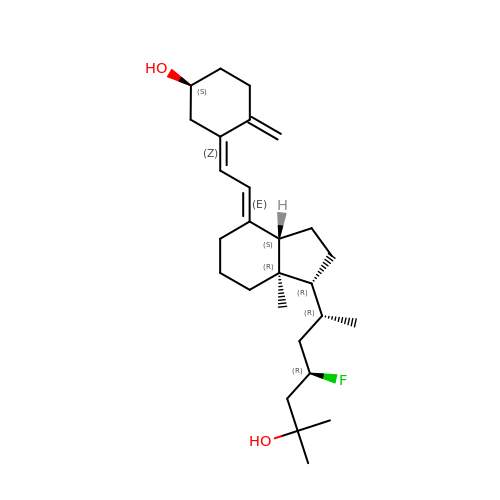(1~{S},3~{Z})-3-[(2~{E})-2-[(1~{R},3~{a}~{S},7~{a}~{R})-1-[(2~{R},4~{R})-4-fluoranyl-6-methyl-6-oxidanyl-heptan-2-yl]-7~{a}-methyl-2,3,3~{a},5,6,7-hexahydro-1~{H}-inden-4-ylidene]ethylidene]-4-methylidene-cyclohexan-1-ol | C27 H43 F O2 | GFRHQHOVEZIWBD-VCAQAZSGSA-N> SLEERVKEIIAEQLGVEKEKITPEAKFVEDLGADSLDVVELIMAFEEEFGIEIPDEDAEKIQTVGDVINYL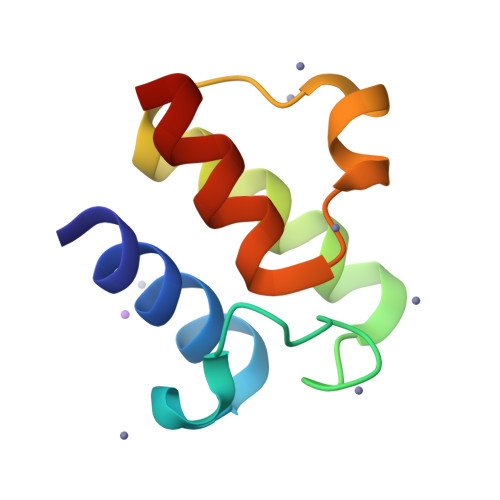KEKVGG> DPV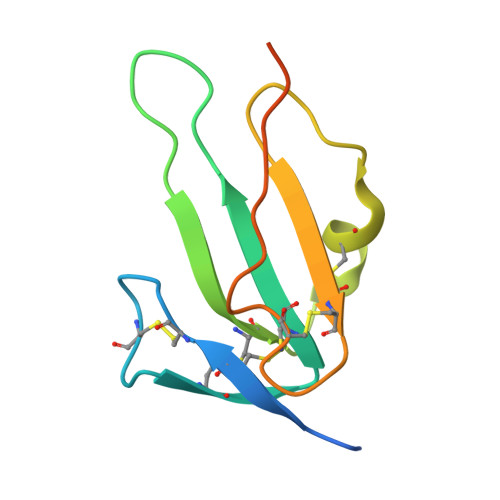KPSRGPLVTCTCESPHCKGPTCRGAWCTVVLVREEGRHPQEHRGCGNLHRELCRGRPTEFVNHYCCDSHLCNHNVSLVLEATQPPSEQPGTDGQ>[4x]MNSNKELMQRRSQAIPRGVGQIHPIFADRAENCRVWDVEGREYLDFAGGQAVLNTGHLHPKVVAAVEAQLKKLSHTCFQVLAYEPYLELCEIMNQKVPGDFAKKTLLVTTGSEAVENAVKIARAATKRSGTIAFSGAYHGRTHYTLALTGKVNPYSAGMGLMPGHVYRALYPCPLHGISEDDAIASIHRIF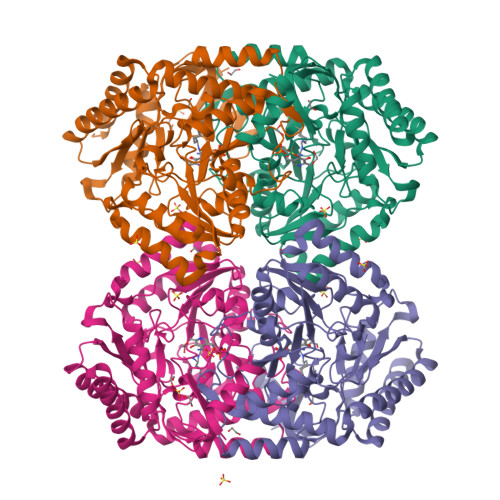KNDAAPEDIAAIVIEPVQGEGGFYASSPAFMQRLRALCDEHGIMLIADEVQSGAGRTGTLFAMEQMGVAPDLTTFAKSIAGGFPLAGVTGRAEVMDAVAPGGLGGTYAGNPIACVAALEVLKVFEQENLLQKANDLGQKLKDGLLAIAEKHPEIGDVRGLGAMIAIELFEDGDHNKPDAKLTAEIVARARDKGLILLSCGPYYNVLRILVPLTIEDAQIRQGLEIISQCFDEAKQ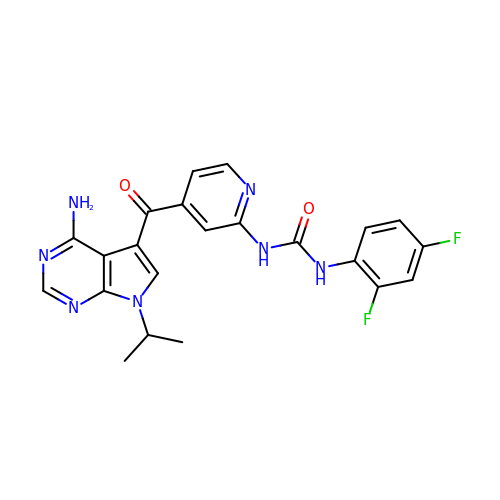N-{4-[4-amino-7-(propan-2-yl)-7H-pyrrolo[2,3-d]pyrimidine-5-carbonyl]pyridin-2-yl}-N'-(2,4-difluorophenyl)urea | C22 H19 F2 N7 O2 | RPNUUULYRBUSBJ-UHFFFAOYSA-N>[3x]PLLERLKRRVVEGRKQGLEADLEEALKAGHKPLDLINGPLLAGMKEVGDLFGAGKMQLPFVLQAAEVMKRAVAYLEPHMEKKGEGKGTLVLATVKGDVHDIGKNLVDIILSNNGYRVVNLGIKVPIEEILKAVEAHKPHAVGMSGLLVKSTLVMKENLEYMRDRGYTLPVILGGAALTRSYVEELRAIYPNVYYAEDAFEGLRLMEELTGHAPPELTRKAPARPKREAPKVAPRARPVGEAPAVPRPPFFGVRVEEGLDLATIAHYVNKLALYRGQWGYSRKGLSREAWQALVEREAEPVFQRLLKEAMAEGWLEPKVLYGFFPVAREGEELLVFSPETGEVLERFRFPRQKGGGLSLVDYFRPRFAA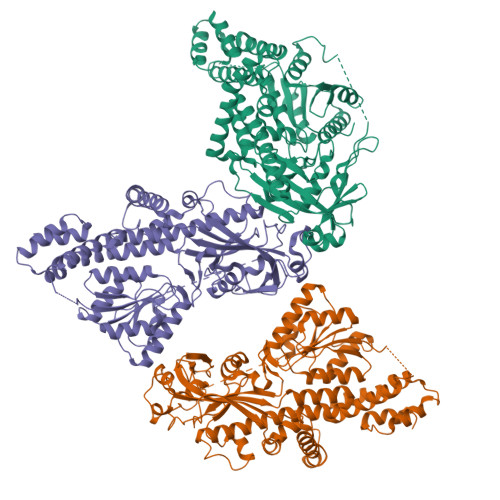PLGDEADWMPKEAFRAGARDVLGVQLVTMGEAPSRKAQALFASGAYQDYLFVHGFSVEMTEALAEYWHKRMRQMWGIAHQDATEIQKLFQQGYQGARYSFGYPACPDLADQAKLDRLMGFHRVGVRLTENFQLEPEHATSALVVHHPEARYFSVD> GSKPFTVPILTVEEMTNSRFPIPLEKLFTGPSGAFVVQPQNGRCTTDGVLLGTTQLSPVNICTFRGDVTHIAGSRNYTMNLASLNWNNYDPTEEIPAPLGTPDFVGKIQGLLTQTTKGDGSTRGHKATVYTGSAPFTPKLGSVQFSTDTENDFETHQNTKFTPVGVIQDGSTTHRNEPQQWVLPSYSGRNVHNVHLAPAVAPTFPGEQLLFFRSTMPGCSGYPNMDLDCLLPQEWVQHFYQEAAPAQSDVALLRFVNPDTGRVLFECKLHK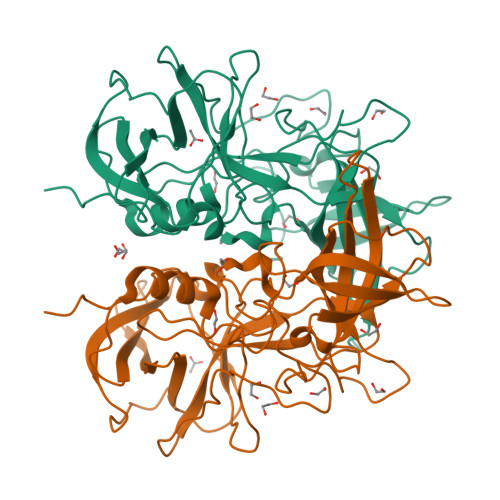SGYVTVAHTGQHDLVIPPNGYFRFDSWVNQFYTLAPM>ALAPMVIEQTSRGERSFDIYSRLLKERVIFLTGQVEDHMANLIVAQMLFLEAENPEKDIYLYINSPGGVITAGMSI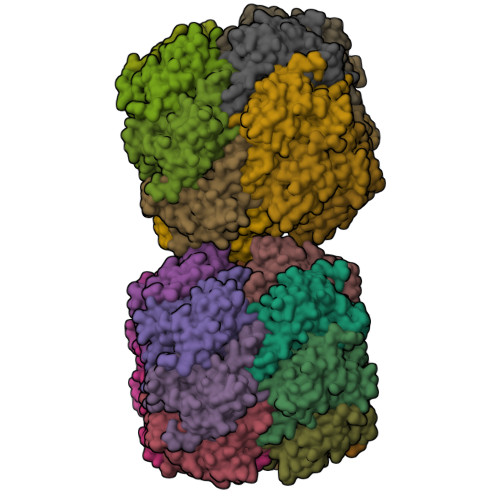YDTMQFIKPDVSTICMGQAASMGAFLLTAGAKGKRFCLPNSRVMIHQPLGGYQGQATDIEIHAREILKVKGRMNELMALHTGQSLEQIERDTERDRFLSAPEAVEYGLVDSILTHRN[28x]> GSSHHHHHHSGDPASMNNHPEVKIKTILSLFLNINIDDFNMDANLADAYDMDXTELADLAKEIEKEFGISVTKSQFSHWETGRAVLDFVSSSLNDKN;>MSEFAMVFPGQGSQDLGMLADLATAFPVVEQTFAEASDVLGYDLWALVQQGPEEELNKTWQTQPALLAASVAIWRVWQEKGGKAPSLMAGHSLGEYSALVCAGVIDFKQAIRLVELRGKLMQEAVPEGTGAMYVIIGLDNESIDRACKEVAQGQIVSPVNFNSPGQVVIAG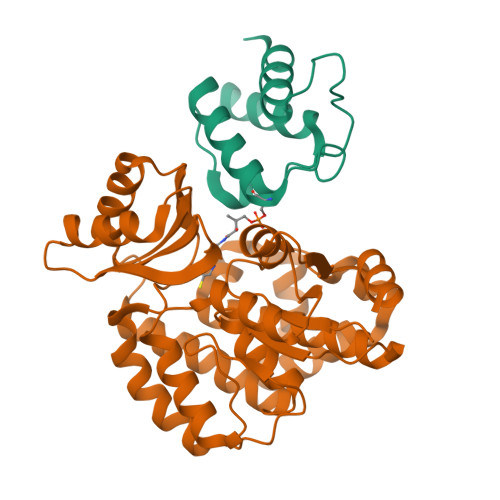EKEAVERAGDACKAAGAKRALPLAVSVPSHCALMKPAADKLAVVLEGIEFGYPQFPVVNNVDVKIEQSAEAIRHALVRQLYNPVRWTETVEFITEQGVGQLLEIGPGRVLTGLTKRIVNTLSAAAVNDTASLITALENN[2x]>MSQDLKLRPLEREDLKFVHELNNNAHIMSYWFEEPYEAFVELQDLYDKHIHDQSERRFIVEKDNEMVGLVELVEIDYIH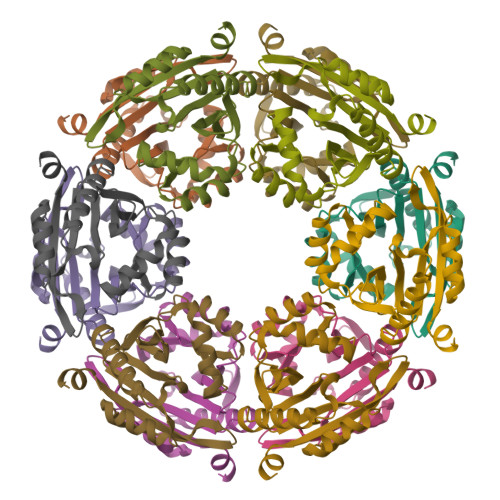RRTEFQIIIDPNYQGYGYAAEATRLAMDYAFSVLNMHKIYLVVDKENEKAVHVYKKVGFMVEGELLDEFFVDGNYHNAIRMCMFQKQYFENK[2x]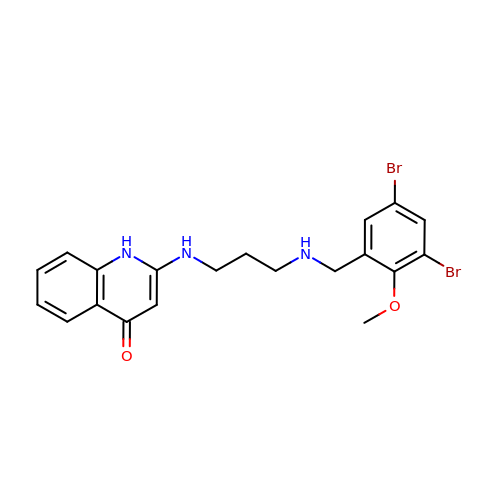2-({3-[(3,5-dibromo-2-methoxybenzyl)amino]propyl}amino)quinolin-4(1H)-one | C20 H21 Br2 N3 O2 | YDCWHIAOHSUPCM-UHFFFAOYSA-N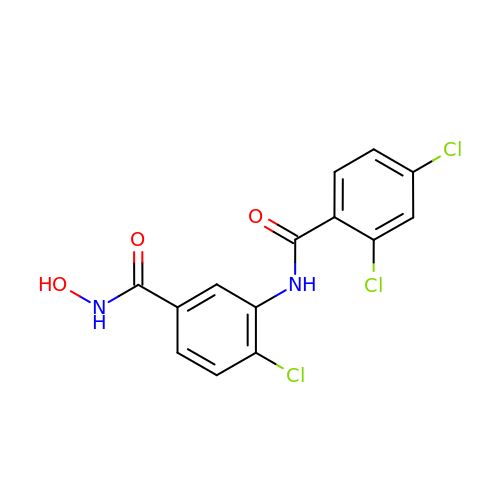4-chloranyl-3-[(2,4-dichlorophenyl)carbonylamino]-~{N}-oxidanyl-benzamide | C14 H9 Cl3 N2 O3 | UYUPOQDZJBPUTQ-UHFFFAOYSA-N>[2x]HHHHHHGSGSTPLKTVRLVGGSGAHEGRVEI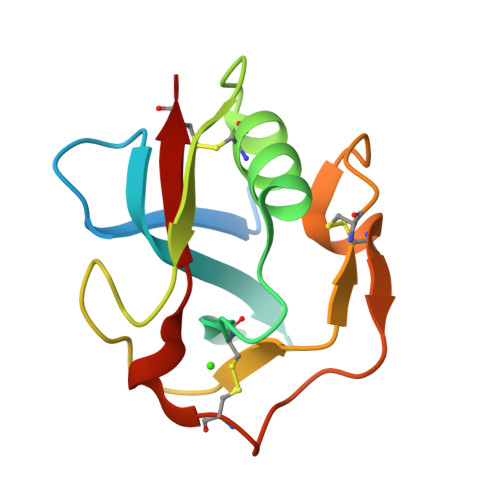FHQGQWGTICDDRWDIRAGQVVCRSLGYQEVLAVHKRAHFGQGTGPIWLNEVMCFGRESSIENCKINQWGVLSCSHSEDAGVTCTS> INQVRPKLPLLKILHAAGAQGEMFTVKEVMHYLGQYIMVKQLYDAAAQHMVYCGGDLLGELLGRQS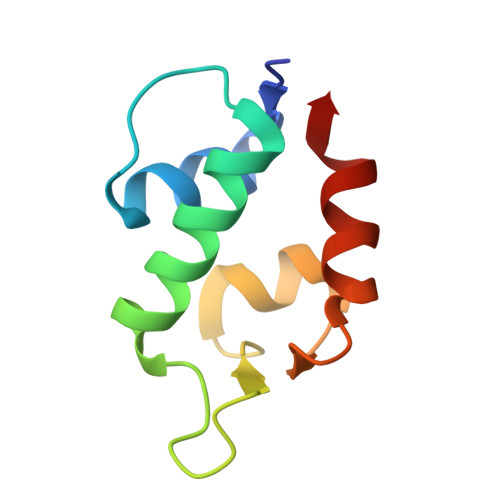FSVKDPSPLYDMLRKNLVT> QGPLGSSEQLKHCNGILKELLSKKHAAYAWPFYKPVDASALGLHDYHDIIKHPMDLSTVKRKMENRDYRDAQEFAADVRLMFSNCYKYNPPDHDVVAMARKLQ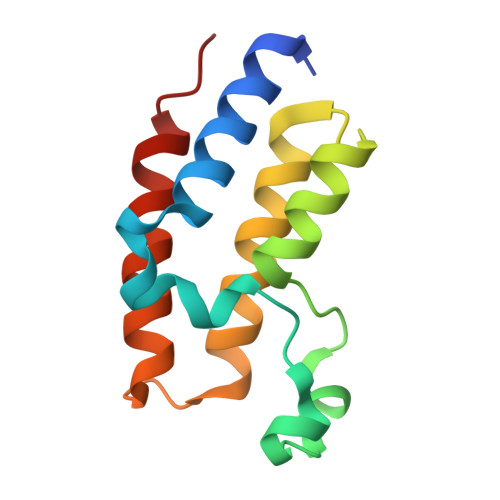DVFEFRYAKMPD> MADPWQECMDYAVTLARQAGEVVCEAIKNEMNVMLKSSPVDLVTATDQKVEKMLISSIKEKYPSHSFIGEESVAAGEKSILTDNPTWIIDPIDGTTNFVHRFPFVAVSIGFAVNKKIEFGVVYSCVEGKMYTARKGKGAFCNGQKLQVSQQEDITKSLLVTELGSSRTPETVRMVLSNMEKLFCIPVHGIRSVGTAAVNMCLVATGGADAYYEMGIHCW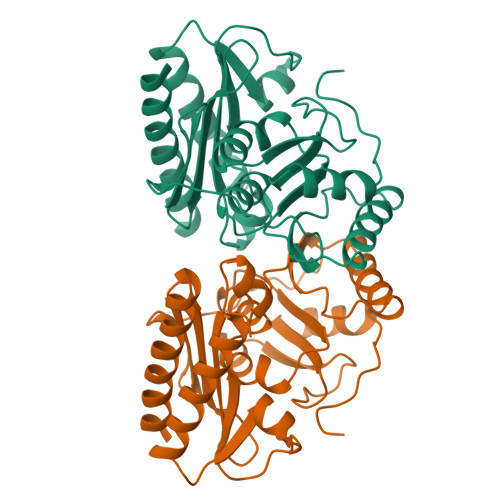DVAGAGIIVTEAGGVLMDVTGGPFDLMSRRVIAANNRILAERIAKEIQVIPLQRDDED> TTGEAYFEQLLDHHNPEKGTFSQRYWWSTEYWGGPGSPVVLFNPGEVSADGYEGYLTNDTLTGVYAQEIQGAVILIEHRYWGDSSPYEVLNAETLQYLTLDQSILDMTYFAETVKLQFDNSSRSNAQNAPWVMVGGSYSGALTAWTESIAPGTFWAYHATSAPVEAIYDFWQYFYPIQQGMAQNCSKDVSLVAEYVDKIGKNGTAKEQQELKELFGLGAVEH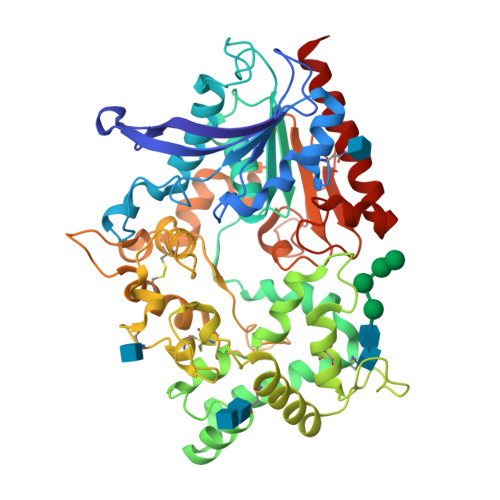YDDFAAVLPNGPYLWQDNDFVTGYSSFFQFCDAVEGVEAGAAVTPGPEGVGLEKALANYANWFNSTILPNYCASYGYWTDEWSVACFDSYNASSPIFTDTSVGNPVDRQWEWFLCNEPFFWWQDGAPEGTSTIVPRLVSASYWQRQCPLYFPEVNGYTYGSAKGKNSATVNSWTGGWDMTRNTTRLIWTNGQYDPWRDSGVSSTFRPGGPLVSTANEPVQIIPGGFHCSDLYMEDYYANEGVRKVVDNEVKQIKEWVEEYYA> MWHYTSINNDTRVALDPKPNQIRTITKPNTVPQLGTDYLYTFNSQRRSHTLRLLGPFQYFNFSETDRGHPLFRLPLKYPSKAIPADELIDNLHSWMRSVHLLHVRSEDNTLRYNWMLGVYARSTNYTTPVGQLVVNAPAILNYSNPQDAFNSVFVALGIDYIDIPITNSNIFDDSSTPYNVRIWHAPTMTEVNHILALMRKSTLVSTHSSWHWNVLHTFHYRSESDMIDHFAAKILEDWRQKEKLDKGALVEADRVIQRLIPLSSSTYVQRLAAIGALYPNEFTENVLDLSRLSTALLQLSDTYYQHANDQLRRLYRRMYNDSRTLYMTQRHQELLLAQITADPNILLYPYTYIFTTIPTSMNYISNTGQGRIKHSLTVTGATEHDTVADIVLGQTGEDVITISMVEPMSIAVEDMYGYVLDTPTRDIWPADEQIEQKGDAVALYDTKTSRALGMFNNTVRIDDLLSPLLSLVYRTYIKGDTMTMTQGSLDHLTLCAAVDSDITFVGNRMIAPLPEGYIPKPMHRNNSTMKMLSLYVALKKLENFATNSYLMAPDTSIILLGAEREPAVNILRRFNRNVSNVRIIGMGDRAVEPNIRVRVPFPIDKNISADFIICDINSYEDQSFESMFSETISVVTTCASAATRALVKINHPSEYMINSVIERLSQLGGVFYHTALLKTASQNPYSYETYIYITPIAAAVRFPFYSNSAMINRYMTAVADDEMPIIPSIHTVIKGHSNTYSPGLFCGCVDVQSAPLALSQLKSYCSEATTWRVDSDDNLVNIIARIDPARIALEFRTRSNTSAYHEYQRYVPNGLGFKVRKTREFRYMHREVTFIHKLMMYALIREQISLTENMTQVVSIGGRNLADISVVPLNMKYVVIDPATRIETLTQEKKNIEVQSRPFQFDAANMDLENNSIYLFIAVIMNEPNGAATPARMQMDKIRNVATAMLTRTNCVAYISFYEAGIITRLDQSTAHKTIRVEEGRLKVANYVPVDTLVEADVTLMLRDIGITHEIIRPSTPELIDACSNYGIRLGSTGGAVLDVFNHYS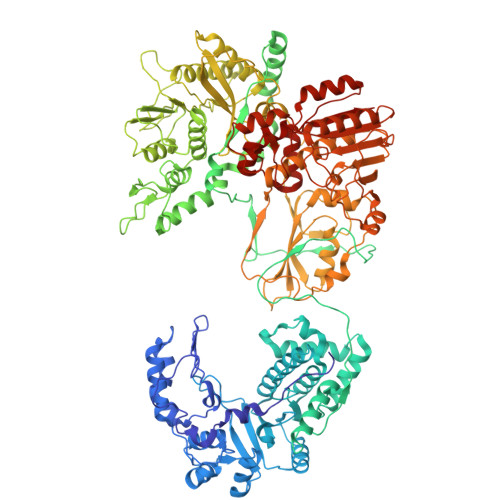PVIKLVRS> MSDKLTRLERLNKEVKKQNKLKQHSKNNRFDDDMDIEAYEDDEQIEEDDFIDDTQEDKKYKKKYREIEDEFDQEIEEEEELNKKKKTKNTILNYTNTTAVTNNKKKAISKQIPDIDIEEIMKLTERKKKIEQEEAQLLQEEQELL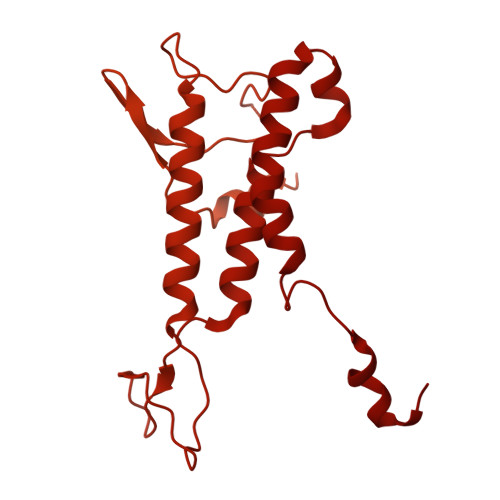EQEKREEEEKKRISQEAKSILREDCASSKTANSSKGKVDQNILNAINRDFSDDSNTVDSISEFQKLKSLAQKANLANESLKQSKVSNTEINLTNLSISQVKKINDYKNEDGSVDAYLYDYFYDAQVKPDKIYAFAKVQNKQTNAFDTCVIQIDTIIRNLFFYPSSDTVTEQQIKNEIAELLKKEQTSRKNVEFLGAFVDKNYAFELPIPRGKSRWYQVVMSYEYEVISPDTKGQYFSYCVGSTYSALETFLITKKITGPSWVRFQNVKDTTSCITNRKLEFRVDYTNQSNIQVLQKQLPTPPLSVVCISLKTSQQIVLSQKKKEYKKEIFNLNMKYHEGINIDNSNKDELNQFKSISFITHIDPTKKQDSITKKGTLPETTKFCLNELNLLEQFLVHFNEIDPDIVVAHDLYSTVFEIILTRIREKGIRKWNLLSKLINIGSSDIPKYGSSTFKTKMAMKGRLLVDTLLSSQEFVNCVEYTLEALAQKLFKIEIPRIDAKAYQQKFATYKLLNSLVDDTYQDIDYALRIMYHLQIVPLTKQLTSICGNIWMGSLQNQRAERNEMLLLHKFNQLNYVYPDNFKNLPESYKKKHKNAQIRKQYEEDEDQAQGNKNPKKKENKYKGGQVFEPEKGLYNEYIVLLDFNSLYPSIIQEFNVCFTTCVRDPIPLEMQMAPFLGNKKAAIQYSKNQNTKENKMQDEDEEDNENEQIVQTHDVLPTIEVIKGIAPLPSILQYLVEQRKVVKNQIKGQKDPQVIETLDIKQKAFKLVANSMYGCLGFSSSRFYAMPLASFITAKGRHILFDSKKIVEDMGYSVIYGDTDSLMIKPGTNEFLEAVKTGLSIKIKVNSKYKKLQLDIDGVFKNMLLLKKKKYATLKVANWEEVKNTNAPEKLEKEIKGIDVVRRDWCQLSRDAGNKILEIILESKSSENMLDDIKKYLIQLNDDINQKNIKNSNYYITKRLTKRVDQYGEKNLPHVAVAQRSIQEKGIDPQTYVNQIISYIICKNEQSSRLVDKAYSPQEFITQSKSLEIDLQYYKRFQLFEPIKRMLEVIEGINLQEIASILEVHYSVQHVSQNNELNAENVLNLKSKRNQFLTSIPRVLVDCKKCDQTFLFLGILEENADAASILKCKCGNDIYIQLKNKIALVVKELIRNFEENAIQIDNEEFEYTHQISLVGKAKQQKMSSFTLNQKLLSIQAMFDITKEEQENTQKVTIEKIKTIKKTLDDLLSKSQYNNLNLSNIFTSFGLLK> SSDSALISGAIVRAFNPERMKVFMHNGCEWLWQAEGTGTRKRAAAHVIIRRGTGQVRVNNDEDLYVRWPFYYNR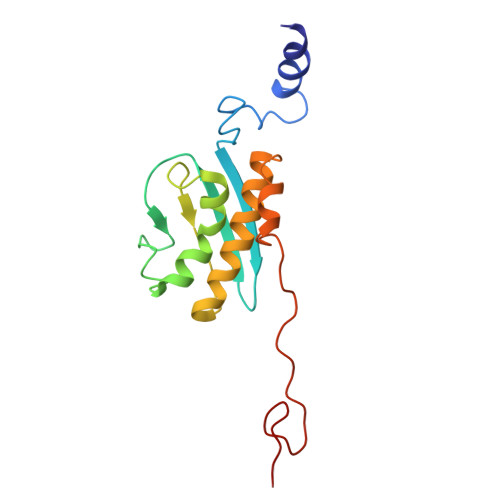MDVLQPFFLTGTAGIYDLFIHVRGGGSSGQAGAVRLAVGRALVSACPACARLLEEDMVLYEDTRQRMPKMPGRMKARKMRTW> MSLTLADKVVYEEEIQKSRFIAKAAPVASEEEALAFLAENREPEATHNGHAYKIGLLYRFSDDGEPSGTAGRPILHAIEAQGLDRVAVLVVRYFGGVKLGAG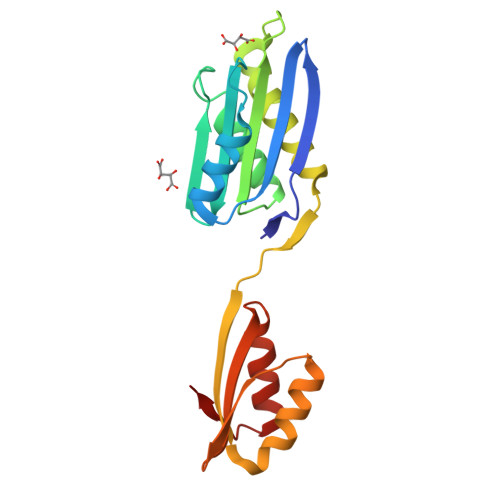GLVRAYGGVAAEALRRAPKVPLVERVGLAFLVPFAEVGRVYALLEARALKAEETYTPEGVRFALLLPKPEREGFLRALLDATRGQVALE> EAQT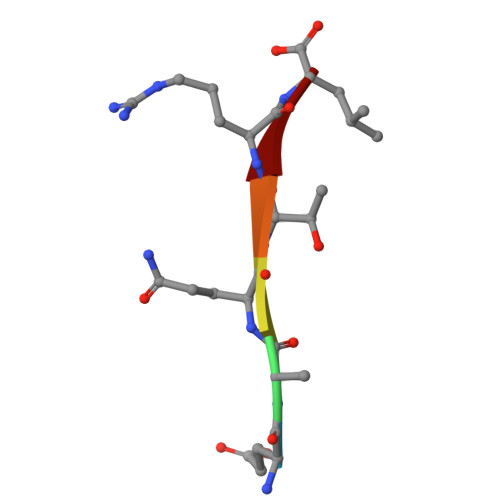RL> S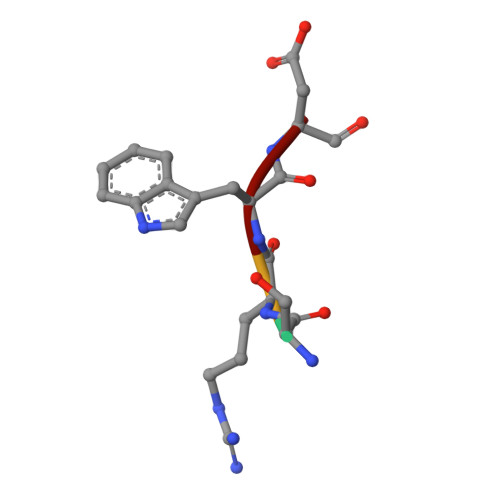RWD> GMPTLEMPVAAVLDSTVGSSEALPDFTSDRYKDAYSRINAIYIEGEQEAHDNYIAIGTLLPDHVEELKRLAKMEMRHKKGFTACGKNLGVEADMDFAREFFAPLRDNFQTALGQGKTPTCLLIQALLIEAFAISAYHTYIPVSDPFARKITEGVVKDEYTHLNYGEAWLKANLESCREELLEANRENLPLIRRMLDQVAGDAAVLQMDKEDL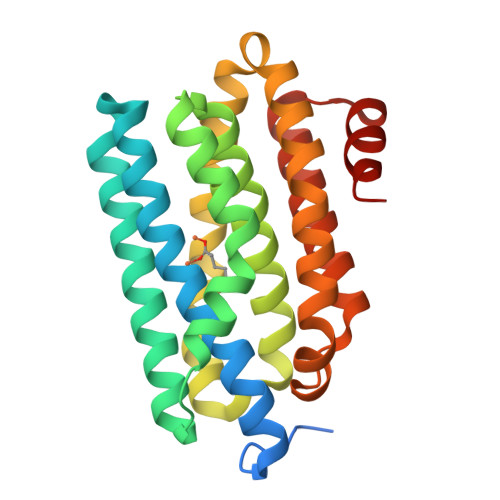IEDFLIAYQESLTEIGFNTREITRMAAAALVS2-[[1-methoxy-4-oxidanyl-7-(4-phenoxyphenoxy)isoquinolin-3-yl]carbonylamino]ethanoic acid | C25 H20 N2 O7 | 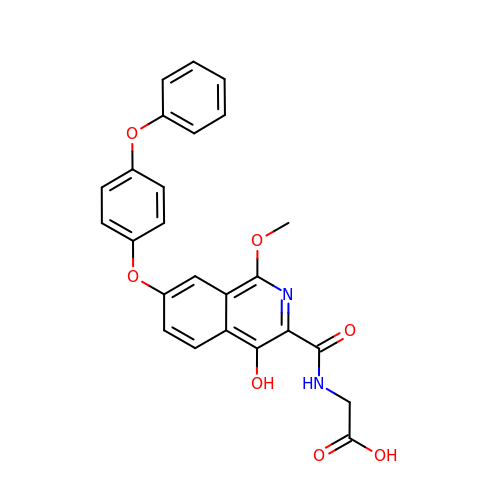NUAFQTOBMYYSNS-UHFFFAOYSA-N Sm and Sm-like (Lsm) proteins have been found in all three kingdoms of life: bacteria, archaea and eukaryotes. They are essential parts of ribonucleoprotein (RNP) complexes and are actively involved in various steps of RNA metabolism including pre-mRNA splicing, mRNA degradation, telomere replication, histone formation and translational control. Members of this protein family are characterized by two closely spaced, conserved Sm motifs 1 and 2, which adopt a conserved Sm fold that consists of an N-terminal α helix followed by a twisted five-stranded β sheet. A common characteristic of Sm/Lsm proteins is their tendency to form a hepta- or hexameric ring structure.

Structure determination of SpLsm2/3 was attempted at a resolution of 2.7 Å. To our surprise, only SpLsm3 was identified in the asymmetric unit (AU). One possibility is that SpLsm2 was lost during crystallization as the crystals were obtained from the heavily precipitated mother liquor. Consistent with this possibility, SDS-PAGE of the protein samples prepared from the thoroughly washed crystals showed that only SpLsm3 was identified in the crystals, thereby confirming that SpLsm2 was precipitated out during crystallization process (Data not shown). The structure of SpLsm3 was solved by single-wavelength anomalous dispersion (SAD) phasing method using a SeMet-substituted crystal. The final model has been refined to an R factor of 24.3% and Rfree of 27.7% with good stereochemical geometry. Residues 1–8 in the N-terminal and residues 56–69 in the loop region are disordered in the electron density map. In the SpLsm3 heptamer, the Lsm3 subunits are assembled one to another to form a heptameric ring via the interactions between strands β4 and β5′ (where ′ indicates the adjacent subunit) in two neighboring subunits. A dimer of heptamers for SpLsm3 observed in the crystal lattices is apparently induced by the crystal packing.

>[14x]MESAQAVAEPLDLVRLSLDEIVYVKLRGDRELNGRLHAYDEHLNMVLGDAEEIVTIFDDEETDKDKALKTIRKHYEMLFVRGDSVILIAPPRN>[4x]GAMELGSLCQGDSMQGQLKLGCIPTIAPFLLCDLVQEINQRFPQLNLLLREDTTTNLLTALRHGELDVLILALPVEIDGMESRVVGQDPFKMV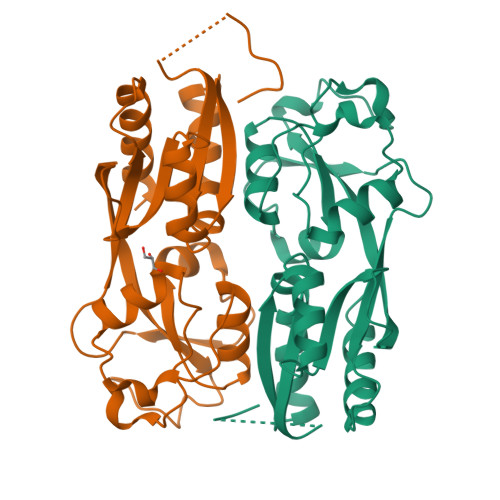ISRHQAGAIKVPIKYDDLPDESVFLLEKGHCLTEHAVSACKLTDKEKINPFSATSLHTLVQMVANGLGTTFIPQMAIDHGLLDNQNLVVIEPPGQQAYRDIGLVWRPSSSRSKTFNQLAEVVSELL> MNSLYELDPKWKKLLKTDNFLGGLTVNEFVQELSKDHRNDVLIDANTKNLPTNEKDQDAIREAIWKQLDPKPYIRTFESTLKELKNLNEETLNKRQYFSEQVATQEVIHSENVIKLSKDLHTTLLTFDKLDDRLTNVTQVVSPLGDKLETAIKKKQNYIQSVELIRRYNDFYSMGKSDIVEQLRLSKNWKLNLKSVKLMKNLLILSSKLETSSIPKTINTKLVIEKYSEMMENELLENFNSAYRENNFTKLNEIAIILNNFNGGVNVIQSFINQHDYFIDTKQIDLENEFENVFIKNVKFKEQLIDFENHSVIIETSMQNLINDVETVIKNESKIVKRVFEEKATHVIQLFIQRVFAQKIEPRFEVLLRNSLSISNLAYVRILHGLFTLFGKFTKSLIDYFQLLEIDDSNQILSTTLEQCFADLFSHYLYDRSKYFGIEKRSLEAILVDMTSKFTVNYDKEINKRVLLDKYKE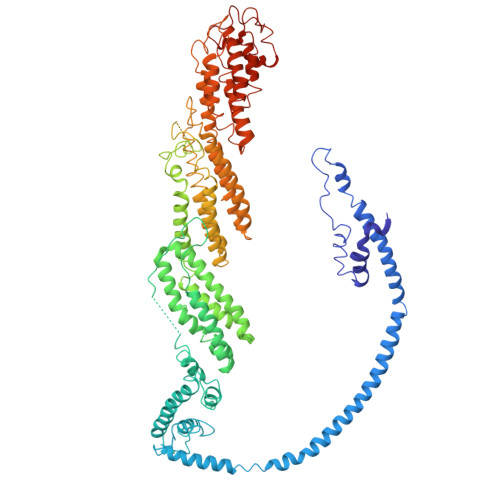KLSTNVDAFMHSPRGNTHSRQDSTSRSKLSQFNSFLKTHLDKDHLSLNRTNTLSDSFNNSSSSTQYDVANNSSSLVNSSFTASDIDNSPNSPANYSLNDVDSMLKCVVESTARVMELIPNKAHLYILEILKIMFLGIVDSYMEIALEVAYWKICKVDINKTAGVVNLNFLKFISMSTEILDLLSISIKSIFLPLLNNSPEIKAQIIEMTNSQIQKMEILINIILQETITVISTKFSAILCKQKKKDFVPKSQELLDQDTLPAIEIVNILNLIFEQSSKFLKGKNLQTFLTLIGEELYGLLLSHYSHFQVNSIGGVVVTKDIIGYQTAIEDWGVASLIDKFATLRELANLFTVQPELLESLTKEGHLADIGRDIIQSYISNREDFNHDNFINSVKLNFR> MAGRLLSRLGLIELGASAACAARQPWPATTTAALPMAVLSALHPWRLAWVTPCGALLLSTSSSSGGAAGATEAVSTSAPFVEPSPSTAAGASAGSSSADIAGPSGDSKPDLVEKLLSSDVLGKGERRRYERQALIREFQRHPADTGSPQVMVAVWTHRVRELVKHFDANRKELRPMRELEIMMNQRRRMLTWLR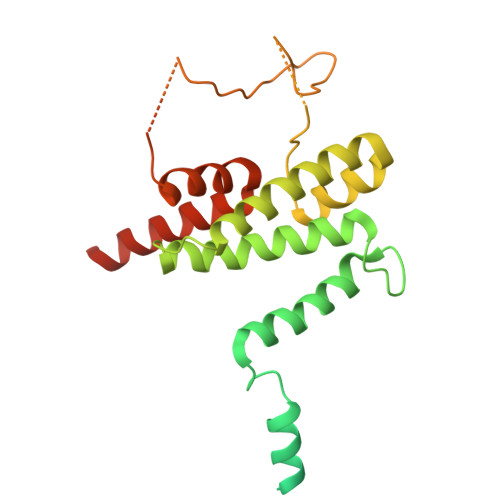RADFESYAYVISKLGLQDIYTSVGISDRYREGLRPSDPVXXXXXXXXXXXXXXXXXXXKDDSVNRLRFNFHKQYKQKKTNLWQRLRPQLLAEDPVLAAQAVATAAAEKQRQTQQRNATSQRLPAQ>[4x]LQAHQDIIANIGEKLGLPLTFDDNNQCLLLLDSDIFTSIEAKDD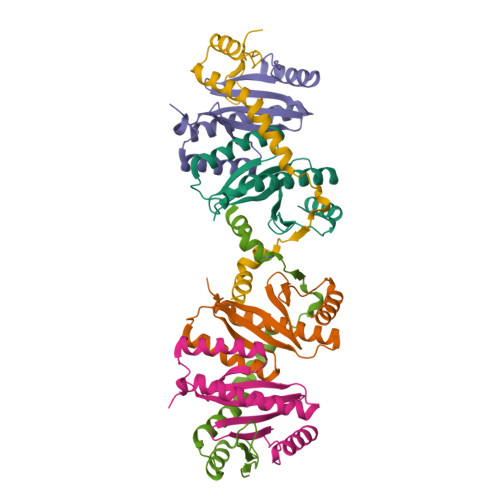IWLLNGMIIPLSPVCGDSIWRQIMVINGELAANNEGTLAYIDAAETLLLIHAITDLTNTYHIISQLESFVNQQEALKNILQEYAKV;>[2x]TDKAYVAPEKFSSKVLTWLGKMPLFKNTEVVQKHTENIRVQDQKILQTFLHALTEKYGETAVNDALLMSRINMNKPLTQRLAVQITECVKAADEGFINLIKSKDN> GSQKQYWVCNSSDASISYTYCDKMQYPISINVNPCIELKGSKGLLHIFYIPRRDLKQLYFN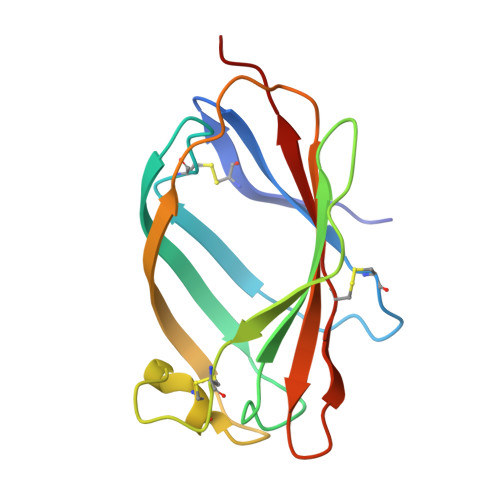LYITVNTMNLPKRKEVICRGSDDDYSFCRALKGETVNTTISFSFKGIKFSKGKYKCVVEAISGSPEEMLFCLEFVILHQPN> NNAFCAGFGLSCKWECWCTAHGTGNELRYATAAGCGDHLSKSYY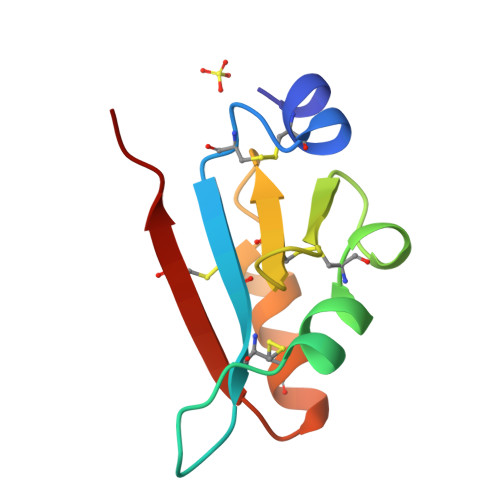DARAGHCLFSDDLRNQFYSHCSSLNNNMSCRSLSK>NGMSEMPAREQMISAYSELVGLDPVSLGDGVAEVRLPMAAHLRNRGGVMHGGA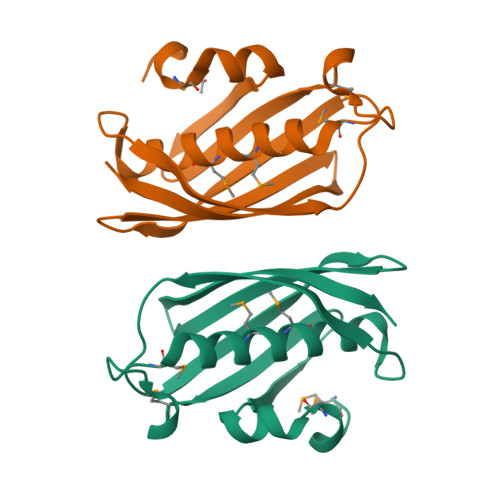LFSLMDVTMGLACSSSHGFDRQSVTLECKINYIRAVADGEVRCVARVLHAGRRSLVVEAEVRQGDKLVAKGQGTFAQLGS[2x]>[2x]MSSVTWAPGNYPSTRRSDHVDTYQSASKGEVPVPDP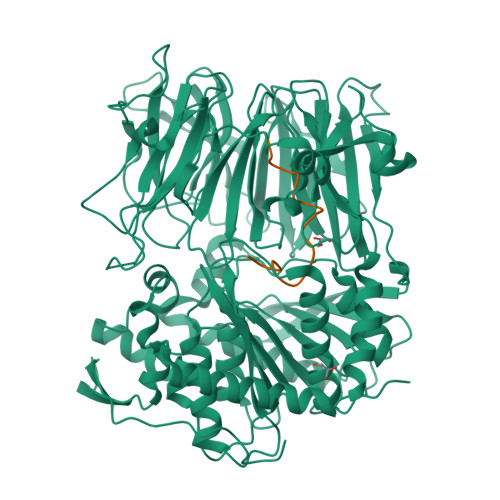YQWLEESTDEVDKWTTAQADLAQSYLDQNADIQKLAEKFRASRNYAKFSAPTLLDDGHWYWFYNRGLQSQSVLYRSKEPALPDFSKGDDNVGDVFFDPNVLAADGSAGMVLCKFSPDGKFFAYAVSHLGGDYSTIYVRSTSSPLSQASVAQGVDGRLSDEVKWFKFSTIIWTKDSKGFLYQRYPARERHEGTRSDRNAMMCYHKVGTTQEEDIIVYQDNEHPEWIYGADTSEDGKYLYLYQFKDTSKKNLLWVAELDEDGVKSGIHWRKVVNEYAADYNIITNHGSLVYIKTNLNAPQYKVITIDLSKDEPEIRDFIPEEKDAKLAQVNCANEEYFVAIYKRNVKDEIYLYSKAGVQLTRLAPDFVGAASIANRQKQTHFFLTLSGFNTPGTIARYDFTAPETQRFSILRTTKVNELDPDDFESTQVWYESKDGTKIPMFIVRHKSTKFDGTAAAIQYGYGGFATSADPFFSPIILTFLQTYGAIFAVPSIRGGGEFGEEWHKGGRRETKVNTFDDFIAAAQFLVKNKYAAPGKVAINGASNGGLLVMGSIVRAPEGTFGAAVPEGGVADLLKFHKFTGGQAWISEYGNPSIPEEFDYIYPLSPVHNVRTDKVMPATLITVNIGAGRVVPMHSFKFIATLQHNVPQNPHPLLIKIDKSWLGHGMGKPTDKNVKDAADKWGFIARALGLELKTVE;>[2x]IWGIGCNPWTAEHVDQTLASGNDIC> MASEAIKGAVVGIDLGTTNSCVAVMEGKQAKVLENAEGARTTPSVVAFTADGERLVGMPAKRQAVTNPNNTFYATKRLIGWRYDDPEVQKDIKNVPFKIVRASNGDAWVEAHGKLYSPSQIGAFVLMKMKETAENYLGHTAKNAVITVPAYFNDSQRQATKDAGQISGLNVLRVINEPTAAALAYGLDKSEDKVIAVYDLGGGTFDISILEIQKGVFEVKSTNGDTFLGGEDFDQALLRHIVKEFKRETGVDLTKDNMALQRVREAAEKAKCELSSSVQTDINLPYLTMDSSGPKHLNMKLTRAQFEGIVTDLIRRTIAPCQKAMQDAEVSKSDIGEVILVGGMTRMPKVQQTVQDLFGRAPSKAVNPDEAVAIGAAIQGGVLAGDVTDVLLLDVTPLSLGIETLGGVFTKLINRNTTIPTKKSQVFSTAADGQTQVEIKVCQGEREMAGDNKLLGQFTLIGIPPAPRGVPQIEVTFDIDANGIVHVSAKDKGTGREQQIVIQSSGGLSKDDIENMVKNAEKYAEEDRRKKERVEAVNMAEGIIHDTETKMEEFKDQLPADECNKLKEEISKMRELLARKDSETGENIRQAASS;>[2x]TLLEEKVKLEEQLKETVEKYKRALADTENLRQRSQKLVEEAKLYGIQAFCKDLLEVADVLEKATQCVPKEEIKDDNPHLKNLYEGLVMTEVQIQKVFTKHGLLKLNPVGAKFDPAEHEALFHTPVEGKEPGTVALVSKVGYKLHGRTLRPALVGVVKEASA;> VLLLDVT

In human mitochondria, mitochondrial Hsp70 (mortalin) and the nucleotide exchange factor (GrpEL1) work synergistically to stabilize proteins, assemble protein complexes, and facilitate protein import. In bacteria, mitochondria, and chloroplasts, the GrpE-family of NEFs interacts with substrate-bound Hsp70 to facilitate ADP and protein substrate release. Herein, we present structures of full-length human mortalin in a nucleotide-free and substrate-bound state in complex with full-length GrpEL1. To stabilize the complex for structural analysis, we introduced a point mutation, R126W, into mortalin (mortalinR126W) that is associated with EVEN-PLUS syndrome and has been shown to reduce mortalin’s ATPase activity and conformational flexibility.

Thus, we mutated Y173 in GrpEL1 to an alanine (GrpEL1Y173A) and performed cryoEM analysis on a mortalinR126W-GrpEL1Y173A complex. Our cryoEM analysis of mortalinR126W-GrpEL1Y173A yielded two distinct populations differentiated by the presence or lack of density for the SBDα lid. We term these structures mortalinR126W-GrpEL1Y173A and mortalinR126W-GrpEL1Y173A−lid. Overall, these structures closely resemble our mortalinR126W-GrpEL1WT structure and are similarly nucleotide-free. Firstly, our mortalinR126W-GrpEL1Y173A structure harbors EM density for the entirety of the SBD, and similar to our mortalinR126W-GrpEL1 structure, appears substrate bound to another mortalinR126W proteolysis product. Critically, we observe a large deviation of the SBD in our mortalinR126W-GrpEL1Y173A structure compared to mortalinR126W-GrpEL1WT, with the SBD of mortalinR126W-GrpEL1Y173A translated ~6 Å away from the GrpEL1-B β-wing. Firstly, positioning of the SBD in our mortalinR126W-GrpEL1Y173A structure suggests that although Y173 in GrpEL1 is not necessary for mortalinR126W-GrpEL1 complex formation, it is key in mediating interaction between the β-wing domain of GrpEL1-B and SBDα lid of mortalin. Secondly, the presence of the full SBD in mortalinR126W-GrpEL1Y173A suggests that interactions between the GrpEL1-B stalk and SBDβ subdomain of mortalin are sufficient in stabilizing the entirety of the SBD. However, the presence of an intact, substrate-bound SBD in our mortalinR126W-GrpEL1Y173A structure suggests that interactions between SBDβ and GrpEL1-B stalk are sufficient to maintain the closed SBD conformation proximal to GrpEL1. We also observe that decoupling the SBD-α:GrpEL1-B interface via Y173A in GrpEL1 results in a change in dynamics only for the GrpEL1-B β-wing.>VQRGYGNPIEASSYGLDLDCGAPGTPEAHVCFDPCQNYTLLDEPFRSTENSAGSQGCDKNMSGWYRFVGEGGVRMSETCVQVHRCQTDAPMWLNGTHPALGDGITNHTACAHWSGNCCFWKTEVLVKACPGGYHVYRLEGTPWCNLRYCTDPSHH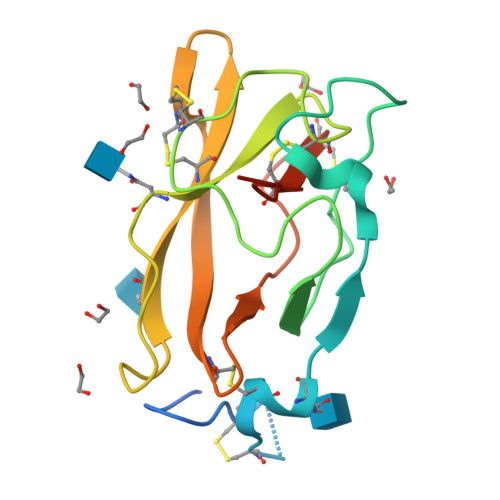HHHHHH[2x]> SNKKTKLIHGGHTTDDYTGAVTTPIYQTSTYLQDDIGDLRQGYEYSRTANPTRSSVESVIATLENGKHGFAFSSGVAAISAVVMLLDKGDHIILNSDVYGGTYRALTKVFTRFGIEVDFVDTTHTDSIVQAIRPTTKMLFIETPSN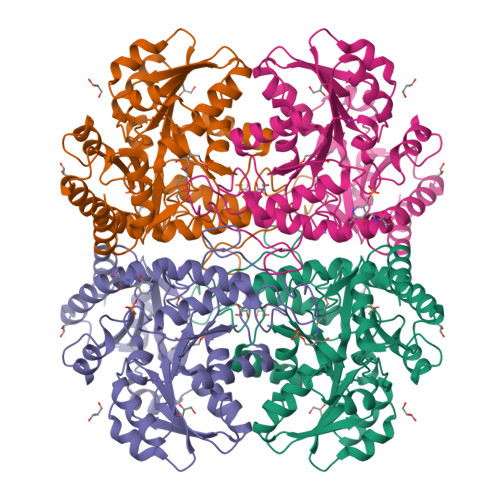PLLRVTDIKKSAEIAKEHGLISVVDNTFMTPYYQNPLDLGIDIVLHSATKYLGGHSDVVAGLVATSDDKLAERLAFISNSTGGILGPQDSYLLVRGIKTLGLRMEQINRSVIEIIKMLQAHPAVQQVFHPSIESHLNHDVHMAQADGHTGVIAFEVKNTESAKQLIKATSYYTLAESLGAVESLISVPALMTHASIPADIRAKEGITDGLVRISVGIEDTEDLVDDLKQALDTL> MKELIYIEEPKILFAHGQKCTDARDGLALFGPLNNLYGIKSGVIGTKQGLKIFRDYLDHIQKPIYNSNSITRPMFPGFEAVFDCKWESTGITFKEVTNEDIGKFLYNSSTHKRTYDLVSLFIDKIISANKNEDENVDVWFVIVPDEIYKYCRPNSVLPKEMVQTKALMSKSKAKSFRYEPSLFPDINIELKEQEKEAETYNYDAQFHDQFKARLLKHTIPTQIFRESTLAWRDFKNAFGLPIRDFSKIEGHLAWTISTAAFYKAGGKPWKLSDVRNGVCYLGLVYKKVEKSKNPRNACCAAQMFLDNGDGTVFKGEVGPWYNPKNGQYHLEPKEAKALLSQSLQSYKEQIGEYPKEVFIHAKTRFNHQEWDAFLEVT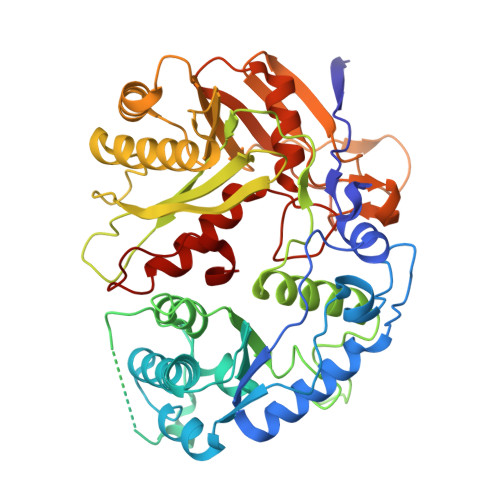PKETNLVGVTISKTKPLKLYKTEGDYTILRGNAYVVNERSAFLWTVGYVPKIQTALSMEVPNPLFIEINKGEADIKQVLKDILSLTKLNYNACIFADGEPVTLRFADKIGEILTASTDIKTPPLAFKYYI>GASAMSLKDKKILIVEDSKFQAKTIANILNKYGYTVEIALTGEA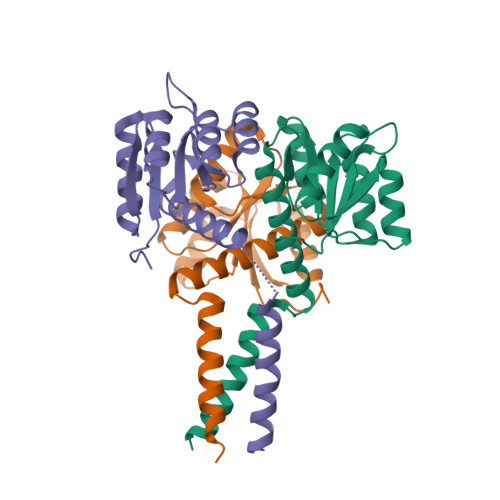AVEKVSGGWYPDLILMDIELGEGMDGVQTALAIQQISELPVVFLTAHTEPAVVEKIRSVTAYGYVMKSATEQVLITIVEMALRLYEANVHANEGSDQDSRLKAIERELEVLTNYVMRS[12x]GlmZ stimulates translation of the mRNA encoding GlcN6P synthtase in Escherichia coli, but when bound by RapZ protein, the sRNA becomes inactivated through cleavage by the endoribonuclease RNase E. Here, we report the cryoEM structure of the RapZ:GlmZ complex, revealing a complementary match of the RapZ tetrameric quaternary structure to structural repeats in the sRNA. RapZ then presents GlmZ to the endoribonuclease RNase E in a manner that directs cleavage within the base‐pairing site of the sRNA, thereby inactivating it and silencing synthesis of the synthase (Göpel et al, 2013; Gonzalez et al, 2017; Durica‐Mitic et al, 2020). The protomers have two domains of roughly equal size: the N‐terminal domain (NTD) bears Walker A and B motifs and resembles an adenylate kinase, while the C‐terminal domain (CTD) bears structural similarity with the sugar‐binding domain of phosphofructokinase. Here, we have elucidated the structures of both the binary complex of RapZ:GlmZ and the ternary complex of the RNase E catalytic domain (RNase E‐NTD), RapZ and GlmZ, using electron cryo microscopy (cryoEM).

To capture a precleavage Michaelis–Menten state of the catalytic domain, the active site residue aspartate 346 in RNase E‐NTD was replaced with cysteine, which changes the metal requirement for ribonuclease activity from Mg2+ to Mn2+ (Thompson et al, 2015). We purified the recombinant mutant RNase E‐NTD, RapZ and GlmZ and combined these components to reconstitute the ternary ribonucleoprotein complex in buffer without Mn2+ but with Mg2+to ensure proper folding of GlmZ and to lock the complex in the precleavage encounter state. The ‘fundamental unit’, comprising one RNase E‐NTD dimer, one RapZ tetramer and one GlmZ RNA (~ 314 kDa) was refined through masking and particle subtraction (Fig EV4), as will be discussed further below. Thus, the interaction of RapZ:GlmZ with RNase E does not involve conformational rearrangement of either RapZ or GlmZ. Previously published crystal and cryoEM structures of RNase E‐NTD have revealed many degrees of freedom at both the quaternary and tertiary levels, enabling flexible accommodation of substrates (Callaghan et al, 2005; Koslover et al, 2008; Bandyra et al, 2012, 2018; Dendooven et al, 2022). It may therefore not be surprising that in the ternary complex structure the 5′‐sensor/S1 domains of the RNase E‐NTD have adopted an opened conformation that can accommodate the binary complex—a configuration not previously observed but which may account for the capacity of RNase E to be guided to preferred cleavage sites by RNA structure. The ternary complex assembly appears to be stabilised predominantly through mutual binding of the RNase E‐NTD and RapZ to GlmZ RNA. The predicted structure of SLIII fits well into the density present on the surface of the RNase E small domain and RNase H fold.

>[4x]MVLMIVSGRSGSGKSVALRALEDMGFYCVDNLPVVLLPDLARTLADREISAAVSIDVRNMPESPEIFEQAMSNLPDAFSPQLLFLDADRNTLIRRYSDTRRLHPLSSKNLSLESAIDKESDLLEPLRSRADLIVDTSEMSVHELAEMLRTRLLGKRERELTMVFESFGFKHGIPIDADYVFDVRFLPNPHWDPKLRPMTGLDKPVAAFLDRHTEVHNFIYQTRSYLELWLPMLETNNRSYLTVAIGCTGGKHRSVYIAEQLADYFRSRGKNVQSRHRTLEKRKP;>[2x]MKRMLINATQQEELRVALVDGQRLYDLDIESPGHEQKKANIYKGKITRIEPSLEAAFVDYGAERHGFLPLKEIAREYFPANYSAHGRPNIKDVLREGQEVIVQIDKEERGNKGAALTTFISLAGSYLVLMPNNPRAGGISRRIEGDDRTELKEALASLELPEGMGLIVRTAGVGKSAEALQWDLSFRLKHWEAIKKAAESRPAPFLIHQESNVIVRAFRDYLRQDIGEILIDNPKVLELARQHIAALGRPDFSSKIKLYTGEIPLFSHYQIESQIESAFQREVRLPSGGSIVIDSTEALTAIDINSARATRGGDIEETAFNTNLEAADEIARQLRLRDLGGLIVICFIDMTPVRHQRAVENRLREAVRQDRARIQISHISRFGLLEMSRQRLSPSLGESSHHVCPRCSGTGTVRDNESLSLSILRLIEEEALKENTQEVHAIVPVPIASYLLNEKRSAVNAIETRQDGVRCVIVPNDQMETPHYHVLRVRKGEETPTLSYMLPKLHEEAMALPSEEEFAERKRPEQPALATFAMPDVPPAPTPAEPAAPVVAPAPKAAPATPAAPAGGEETKPTEQPAPKA> MSQRITIDPVTRIEGHLRIDCEIENGVVSKAWASGTMWRGMEEIVKNRDPRDAWMIVQRICGVCTTTHAISSVRAAESALNIDVPVNAQYIRNIILAAHTTHDHIVHFYQLSALDWVDITSALKADPAKASAMLNGVSTWHLNSAEEFTKVQNKIKDLVASGQLGIFANGCWGHPAMQLPPEVNLIAVAHYLQALECQRDANRVVALLGGKTPHIQNLAVGGVANPINLDGLGVLNLERLMYIKSFIDKLSDFVEQVYKVDTAVIAAFYPEWLERGQGAVNYLSAPEFPTDGKNGSFLFPGGYITDADLSTYRPITSHSDEYLIKGIQESAKHAWYKDEAPQAPWEGTTVPDYTGWSDDGKYSWVKAPTFYGKTVEVGPLANMLCKLAAKRESTHAKLNEIVAIYTKLTGKTIEVAQLHSTLGRIIGRTVHCCELQNVLQDQYN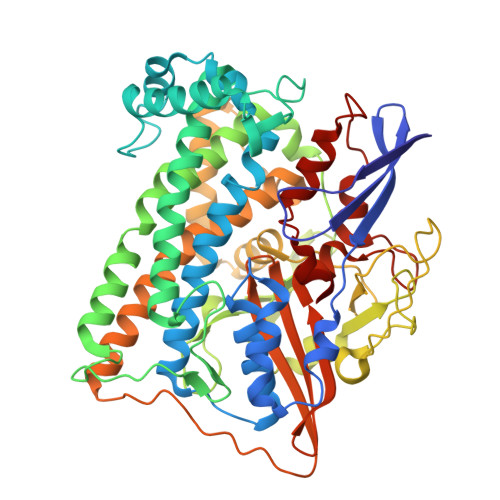ALIVNIGKGDHTTFVKPDIPATGEFKGVGFLEAPRGMLSHWMVIKDGIISNYQAVVPSTWNSGPRNFNDEVGPYERSLVGTPIADPNKPLEVVRTIHSFDPCMSCAVH>MTTQKPADFPYPSHFADVLGSRMHYVEHGNGDPLLFLHGQPTWSYLWRKVL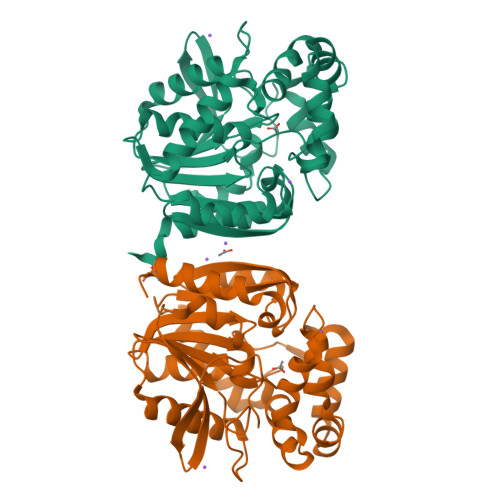PELEGKGRLIAVDLIGYGMSDKPDIPYDIDDHIRYLDGFIEALGLDRITIVCHDWGSFFGFHYAHRHPERIKGLAFMEAMLNPIPGYDAFDPQTRAFFQTLRSSQANAERMMMDENQFVENILPAMICRPLERQELDAYRAPWTDRQSRRILCTFPQNLCIGKEPASVYRMQTAYIEWLGQTDLPKLLIHAEPGFLIPAPAVDQYRQQLPNLETAFVGSGLHYIQEDQPQKIGQAIAQWMDRCGLHHHHHH[2x]(2R)-3-{[(4Z)-5,6-DIPHENYL-6,7-DIHYDRO-4H-PYRROLO[2,3-D]PYRIMIDIN-4-YLIDENE]AMINO}PROPANE-1,2-DIOL 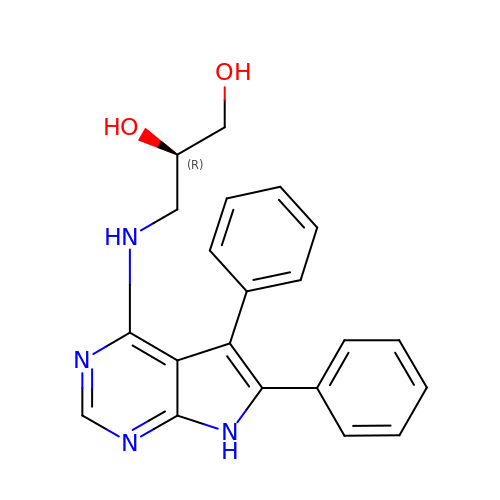| C21 H20 N4 O2 | TWEONIHFGKSPLC-MRXNPFEDSA-N(4S,8E,11R)-4-[(1R)-1-hydroxy-2-{[3-(propan-2-yl)benzyl]amino}ethyl]-16-methyl-11-phenyl-6-oxa-3,12-diazabicyclo[12.3.1]octadeca-1(18),8,14,16-tetraene-2,13-dione | C34 H41 N3 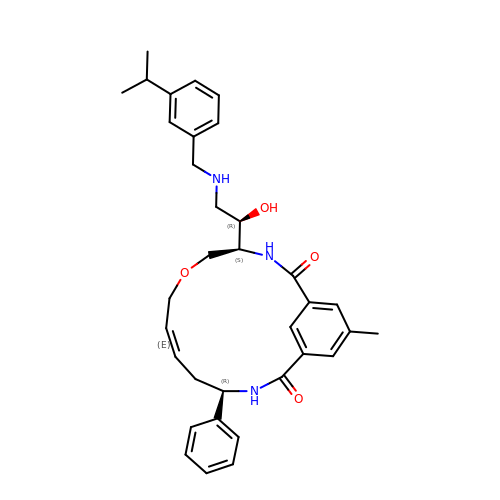O4 | BEGCWPHKTGGGNN-HOQOQLLYSA-N>[12x]MSL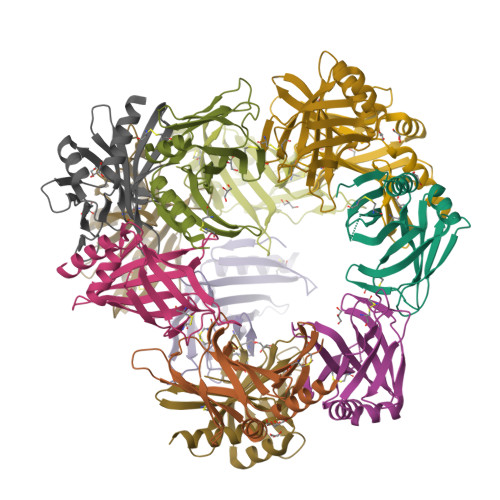SNSKSTTTKDTVATLPNGASSLTETYGLWSINCGIQEGKKVCFMHRQEVNDQNRVVVAMSVVLNADGVVSGNLTVPFGILVSKPVRLQVDEGKAVIETGIRTCVPAGCIVPIVFDKNYVAALRAGKHLKLAMTIAAPGEPPLNDLFVQLNGFSNALNRLIALQKEGHHHHHH>GKSPTEVLLELIAEASGTTREEVKEKFLKELRKGKSPTEVLLELIAEASGTTKEEVKEKF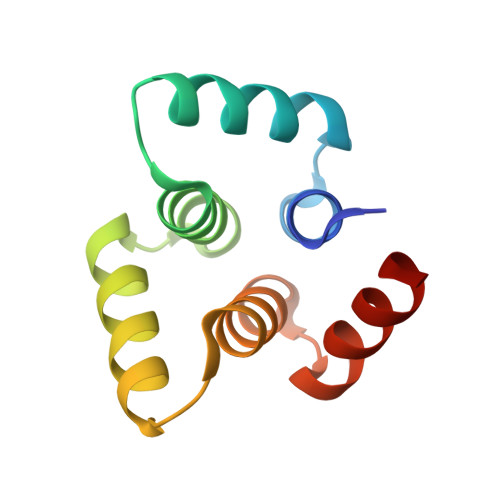LKELSFGKSPTEVLLELIAEASGTTKEEVKKKFWKELSL[2x]> MTMDEKYVNSIWDLLKNAIQEIQRKNNSGLSFEELYRNAYTMVLHKHGEKLYTGLREVVTEHLINKVREDVLNSLNNNFLQTLNQAWNDHQTAMVMI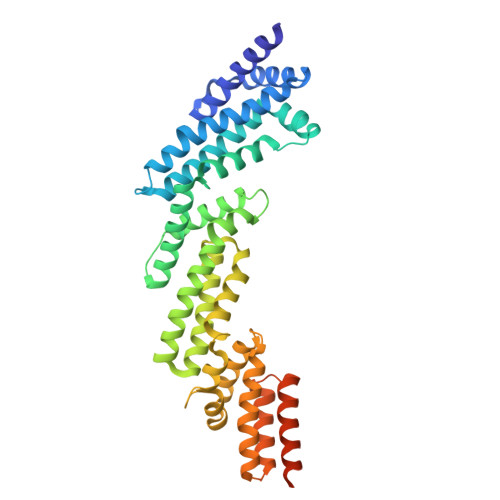RDILMYMDRVYVQQNNVENVYNLGLIIFRDQVVRYGCIRDHLRQTLLDMIARERKGEVVDRGAIRNACQMLMILGLEGRSVYEEDFEAPFLEMSAEFFQMESQKFLAENSASVYIKKVEARINEEIERVMHCLDKSTEEPIVKVVERELISKHMKTIVEMENSGLVHMLKNGKTEDLGCMYKLFSRVPNGLKTMCECMSSYLREQGKALVSEEGEGKNPVDYRQGLDDLKSRFDRFLLESFNNDRLFKQTIAGDFEYFLNLNSRSPEYLAENLYFQSHHHHHHDYKDDDDK> LAPSPQSPETPAPQNQTSRVVQAPKEEEEDEQEASEEKASEEEKAWLMASRQQLAKETSNFGFSLLRKISMRHDGNMVFSPFGMSLAMTGLMLGATGPTETQIKRGLHLQALKPTKPGLLPSLFKGLRETLSRNL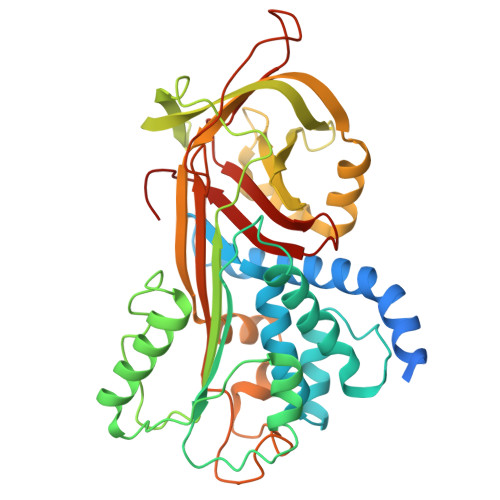ELGLTQGSFAFIHKDFDVKETFFNLSKRYFDTECVPMNFRNASQAKRLMNHYINKETRGKIPKLFDEINPETKLILVDYILFKGKWLTPFDPVFTEVDTFHLDKYKTIKVPMMYGAGKFASTFDKNFRCHVLKLPYQGNATMLVVLMEKMGDHLALEDYLTTDLVETWLRNMKTRNMEVFFPKFKLDQKYEMHELLRQMGIRRIFSPFADLSELSATGRNLQVSRVLQRTVIEVDERGTEAVAGILSEITAYSMPPVIKVDRPFHFMIYEETSGMLLFLGRVVNPTLL>[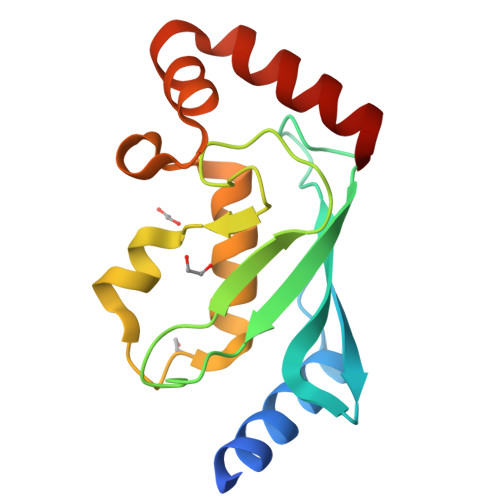2x]MNSNVENLPPHIIRLVYKEVTTLTADPPDGIKVFPNEEDLTDLQVTIEGPEGTPYAGGLFRMKLLLGKDFPASPPKGYFLTKIFHPNVGANGEICVNVLKRDWTAELGIRHVLLTIKMLLIHPNPESALNEEAGRLLLENYEEYAARARLLTEIHG> PTVEYLNYEVVDDNGW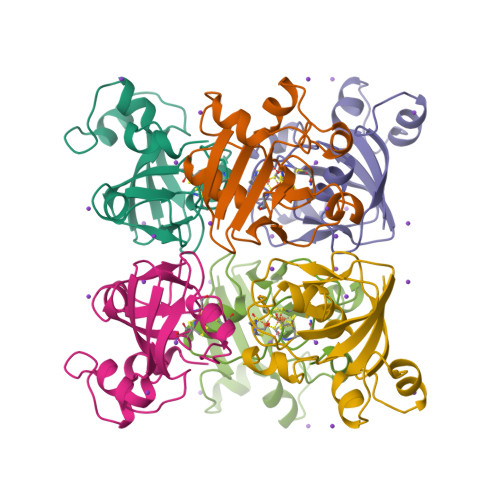DMYDDDVFGEASDMDLDDEDYGSLEVNEGEYILEAAEAQGYDWPFSCRAGACANCAAIVLEGDIDMDMQQILSDEEVEDKNVRLTCIGSPDADEVKIVYNAKHLDYLQNRVI The human assembly factor Coa6 participates in the biogenesis of the CuA site in complex IV (cytochrome c oxidase, COX). Coa6 is a soluble IMS protein with a CX9C–CX10C sequence motif, which binds Cu(I) with a KD(CuI) of ∼10−17 M. Coa6 deletion in both yeast and human cells results in diminished COX assembly and activity; however, this defect can be partially rescued by exogenous copper supplementation and in yeast by treatment with elesclomol (via a proposed elesclomol–copper complex). Here, we present the crystal structures of human Coa6 and the pathogenic W59CCoa6-mutant protein. These structures show that Coa6 has a 3-helical bundle structure, with the first 2 helices tethered by disulfide bonds, one of which likely provides the copper-binding site. Patients with mutations in Coa6 suffer from mitochondrial disease due to complex IV deficiency.

To elucidate the atomic structure of the WTCoa6 protein, we crystallized and determined its structure to 1.65 Å resolution by X-ray crystallography. The structure shows two monomers of WTCoa6 per asymmetric unit, arranged as an antiparallel dimer. Each monomer is composed of a 3-helical bundle, with a coiled–coil–helix–coiled–coil–helix (CHCH) fold. The sequence of WTCoa6 includes four Cys residues (at positions 58, 68, 79, and 90) in a CX9C–CX10C sequence motif, which in the crystal structure form two intramolecular disulfide bonds per monomer, between Cys58–Cys90 and Cys68–Cys79, in accordance with the fully oxidized state of the protein. These disulfides tether helices α1 and α2 together at each end of the helical pair. The Coa6 dimer has buried surface areas of 701 and 656 Å2 (for molecules A and B, respectively), which are 15 and 13%, of the total surface areas of each corresponding monomer, indicating that WTCoa6 forms a stable dimer in solution. The Coa6 dimer is entirely mediated by intermolecular contacts between Helix α3 from each monomer. In addition, Tyr97 of monomer A (Helix α3, cyan) forms a π-stacking interaction with Phe111 of monomer B (Helix α3, gray) at the dimer interface. Interestingly, an analysis of the geometries and potential energies of the Cys58–Cys90 and Cys68–Cys79 disulfides revealed that the Cys58–Cys90 bond has a +/−RHHook geometry, which is commonly observed for disulfide bonds within thioredoxin-like proteins,beeing classified as a “catalytic” conformation. In addition, the structure of WTCoa6 shows that the Cys58–Cys90 site is proximate to positively charged residues (Lys53 and Arg55) and bordered by aromatic side chains (Trp59 and Trp94), which partially shield the site from the solvent.

>[2x]PSMKERQVCWGARDEYWKCLDENLEDASQCKKLRSSFESSCPQQWIKYFDKRRDYLKFKEKFEAGQFEPS>GPMETAQYSTSKTPYSPQQDIRTYQPPPPGFTAVFTELVSRHGSRTPTKIDGADLLLQLWAKARDESELTSAGQDFGPTMESYRAAIQKVGLGQETGRGRQELQGMADRMQRRLPELFEKIKKDATPIAVVLSQQTGRIADTAKFFTARLGATDPALAPLIQQPVVDQDLLYFHKTERGKAYRDYLENDQRYQETVKRIKNRDGTREAATDILKTIFTPAFVERMEPSAVTKAAQALYDLDAIAPDLSVEGNWHLDRFVPRHAAAWFASIDDAKSFYKKGPGFEGSDITFAMASILLDDFFKQAEAARAGKLGADLRFTHAEEIIPLAALMQLPGSEKQADPDEDYTYANNPWR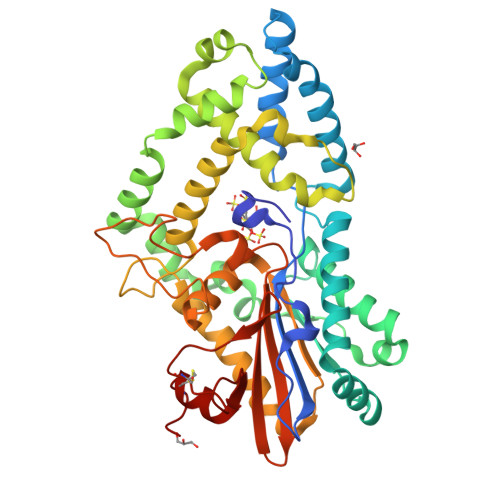GASVSPMAANLQWDIYRNGTTYLVRMLYQEKEIPFKPDCTPFTPGSHYYRLDELSRCFGRTAR[2x]> MLLKRLGLATLLSFSVVGCTTAPNTLAINTTQKIIQYERSKSDLTTQSFTLSSGDKIVYAENGNVAGEPLLLVHGFGGNKDNFTRIARQL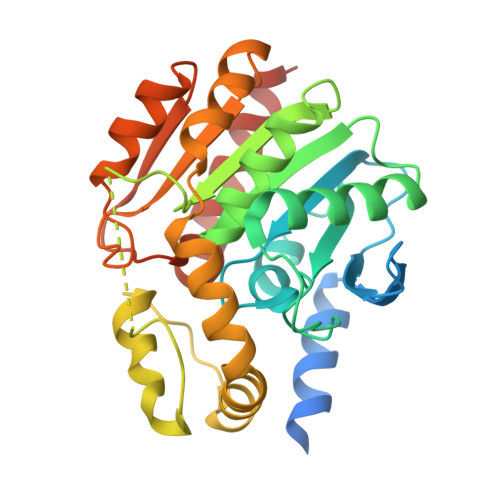ENYNLIIPDLLGFGDSSKPMAADYHSEAQATRLHELLQAKGLASSIHVGGNSMGGAISVAYAAKYPKEVKSLWLIDSAGFWSAGVPKSLESATLENNPLLVDKKEDFYAMYDFVMSKPPYIPKSVKAVFAQERIANKALESKILAQIVEDNVEQRAKVITEYNIPTLVVWGEEDKVIKPETVTLIKEIIPQSQVITMPKIGHVPMIEAVKDTANDYKAFREGLKNVEHHHHHH>[2x]KAPSQNAIKRFMTLFSGREDVFSIQYEGGYRPIRRPLNFQDIKNHFSGKKTLGIYLLKKNDTVKFAAYDIDIKKHYLNREDKF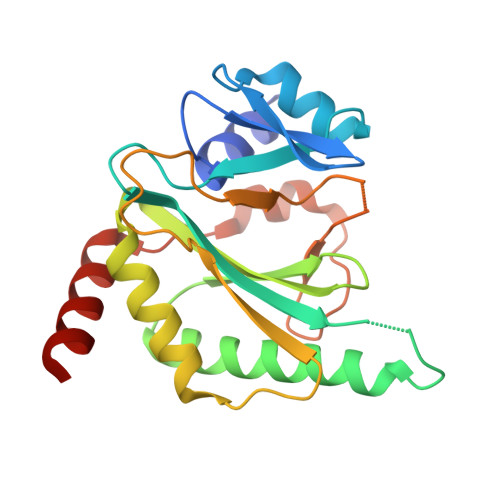VYEENSKKVAKRLSRELNLENITHYFEFTGNRGYHIWIFFDIPVSAYKIKYIMEKILDRIELEEGIDVEIFPKQTSLNGGLGNLIKVPLGVHKKTGKKCLFVDNDFNVIENQIEFLNNIKENKATEINKLFREIFNEND2-cyclopropyl-N-{5-[4-({5-[(cyclopropylacetyl)amino]-1,3,4-thiadiazol-2-yl}oxy)piperidin-1-yl]-1,3,4-thiadiazol-2-yl}acetamide 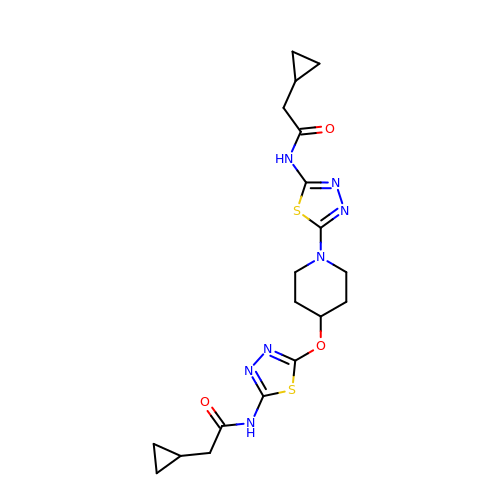| C19 H25 N7 O3 S2 | JHCGNAVCXZTYNC-UHFFFAOYSA-N N-(1,3-benzothiazol-2-yl)-2-(4-{[(4-{[(2R)-4-(morpholin-4-yl)-1-(phenylsulfanyl)butan-2-yl]amino}-3-[(trifluoromethyl)sulfonyl]phenyl)sulfonyl]carbamoyl}-1,3-thiazol-2-yl)-1,2,3,4-tetrahydroisoquinoline-8-carboxamide | C42 H40 F3 N7 O7 S5 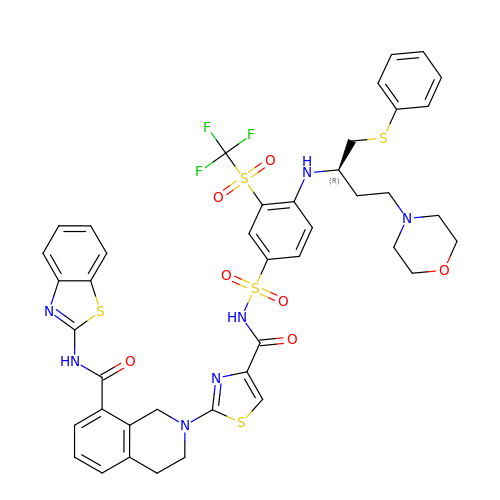| GSXZYBFDAFXVFZ-MUUNZHRXSA-N> MPLAGSELPRRPLPPAAQERDAEPRPPHGELQYLGQIQHILRCGVRKDDRTGTGTLSVFGMQARYSLRDEFPLLTTKRVFWKGVLEELLWFIKGSTNAKELSSKGVKIWDANGSRDFLDSLGFSTREEGDLGPVYGFQWRHFGAEYRDMESDYSGQGVDQLQRVIDTIKTNPDDRRIIMCAWNPRDLPLMALPPCHALCQFYVVNSELSCQLYQRSGDMGLGVPFNIASYALLTYMIAHITGLKPGDFIHTLGDAHIYLNHIEPLKIQLQREPRPFPK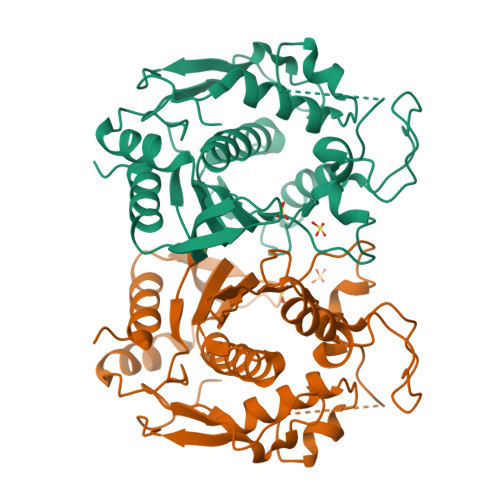LRILRKVEKIDDFKAEDFQIEGYNPHPTIKMEMAV> QFAKPEDAVKYRQSALTLMASHFGRMAPVVKGQAPYDAAQIKANVEVLKTLTALPWAAFGAGTEGGDARPEIWSDAAGFKQKQQAFQDNIVKLSAAADAGDLDKLRAAFGDVG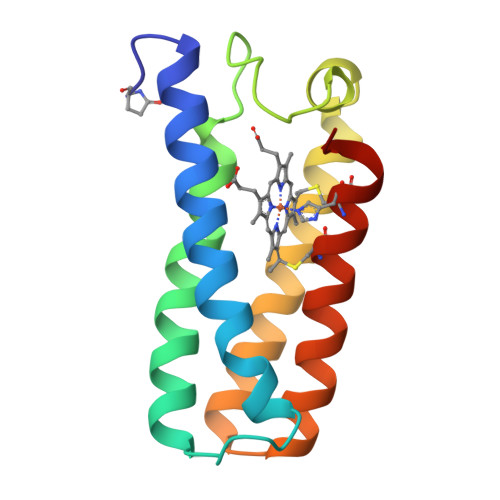ASCKACHDSYRKKK>[15x]ENSGGNAFVPAGNQQEAHWTINLKDADIREFIDQISEITGETFVVDPRVKGQVSVVSKAQLSLSEVYQLFLSVMSTHGFTVVAQGDQARIVPNAEAKTEAGGGQSAPDRLETRVIQVQQSPVSELIPLIRPLVPQYGHLAAVPSANALIISDRSANIARIEDVIRQLDQKGSHDYSVINLRYGWVMDAAEVLNNAMSRGQAKGAAGAQVIADARTNRLIILGPPQARAKLVQLAQSLDTPTARSANTRVIRLRHNDAKTLAETLGQISEGMKNNGGQGGEQTGGGRPSNILIRADESTNALVLLADPDTVNALEDIVRQLDVPRAQVLVEAAIVEISGDIQDAVGVQWAINKGGMGGTKTNFANTGLSIGTLLQSLESNKAPESIPDGAIVGIGSSSFGALVTALSANTKSNLL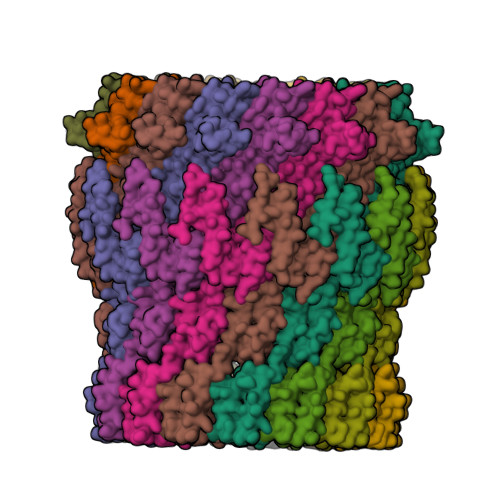STPSLLTLDNQKAEILVGQNVPFQTGSYTTNSEGSSNPFTTVERKDIGVSLKVTPHINDGAALRLEIEQEISALLPNAQQRNNTDLITSKRSIKSTILAENGQVIVIGGLIQDDVSQAESKVPLLGDIPLLGRLFRSTKDTHTKRNLMVFLRPTVVRDSAGLAALSGKKYSDIRVIDGTRGPEGRPSILPTNANQLFDGQAVDLRELMTE>MSLKRYRTLLFDVDDTILDFQAAEALALRLLFEDQNIPLTNDMKAQYKTINQGLWRAFEEGKMTRDEVVNTRFSALLKEYGYEADGALLEQKYRRFLEEGHQLIDGAFDLISNLQQQFDLYIVTNGVSHTQYKRLRDSGLFPFFKDIFVSEDTGFQKPMKEYFNYVFERIPQFSAEHT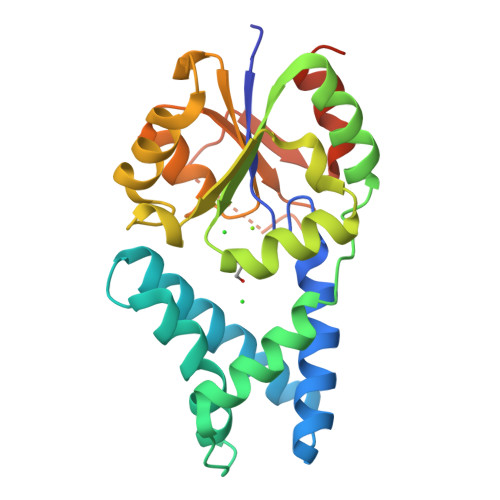LIIGDSLTADIKGGQLAGLDTCWMNPDMKPNVPEIIPTYEIRKLEELYHILNIENTVSEGHHHHHH[3x]>MVKGTPGNVPAARTGIEITAAHRAFFHALPKVELHCHLLGAVRHDTFVALAQRSGAPIERAEIDAFYARGEKPVGVLHVLRALDRYLLTRPDDLRRIAYEYLEDAAAHNVRHAEFFWNPTGTVRVSGIPYADAQAAIVTGMRDAARDFGIGARLIPSIDREQDPDEAVAIVDWMKANRADEVAGIGIDYRENDRPPELFWKAYRDARAAGFRTTAHAGEFGMPWRNVETAVDLLHVDRVDHGYTIVDNPELCARYAER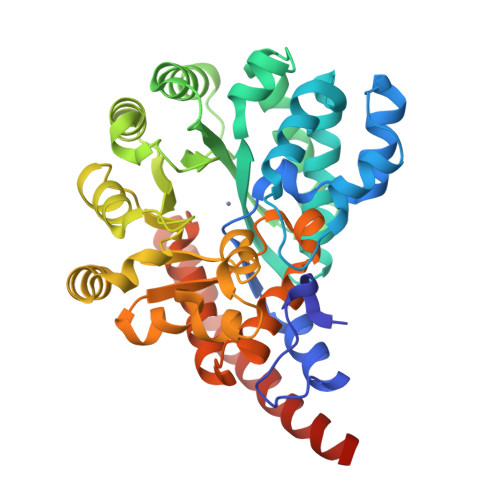GIVFTVVPTNSYYLRTLPPDQWAERHPMRKMPGLGLKIHPNTDDPTLHKVNPSEAWELMFSHFGFTIADLKQFMLNGIDGAWVDDDTKAAWRAAWAPEFDMLADTLAADKLAAALEHHHHHH[2x]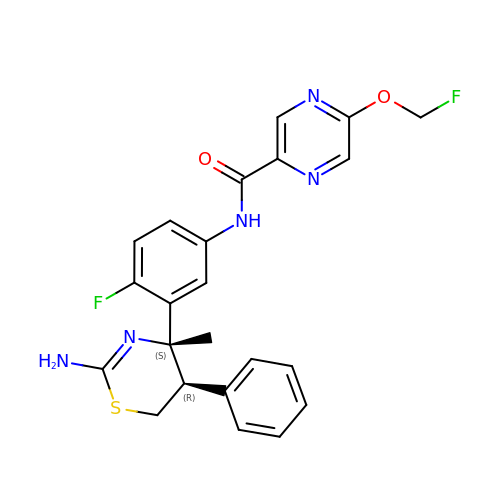N-[3-[(4S,5R)-2-azanyl-4-methyl-5-phenyl-5,6-dihydro-1,3-thiazin-4-yl]-4-fluoranyl-phenyl]-5-(fluoranylmethoxy)pyrazine-2-carboxamide | C23 H21 F2 N5 O2 S | BCDWEYSMCDBNJS-UZUQRXQVSA-N>[2x]GMRPGSSERNHPAERPTTILSGSMAPAAVPHVALLPSSGMG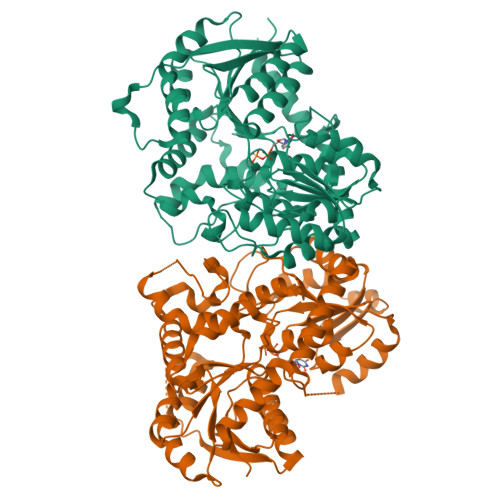HLTPFLRLAAALASHGCVITFITPTPVVSAAEARHVEAFISSSPLFRRLEFPLLPFDVSSVVSDDPFFLQFERISRSARHLGPVLSSVSPPLSALILDVTLTSSILPIAAEISLPAYILFTSSAGMLSLCLSYPEIAASGGVTIKIPGVAEDLAPSSLPQPLRDPRNLFTGQFIENGRAMARADGIIINTWEALEPATLAALQGSKAVSGFPLVIPVGPLLAASDIHTAADDLVIPWLDAQPASSVVFVSFGSRTALSAEQLRELAAGLESSGCRFLWVLKTKKVDREDQEGEKAVDELLGEGFLQRVEWKGKVVSGWVDQRAVLDHPSVGGFVSHCGWNSVTEAALGGMRVLAWPRHGDQRINAMVVEKSGLGKWPSLWTWEGDDEIVRREEIAGRVAELMASPAAAAAAAKVKEEAVRAATAGGSSQRQLEDLVSRFTCSGD Here, we addressed the problem of accurate structural validation with cryo-EM-based methodologies for determining the structures of up to megadalton-scale DNA objects in solution, together with molecular-dynamics-based methods for building pseudoatomic models in a semiautomated fashion. The library of objects includes four brick-like multilayer DNA origami objects with increasing internal floppiness, a barrel-like 126-helix bundle, two variants of a multidomain object called Twisttower, a design variant v2 of a previously reported object called the Pointer, a small 16-helix bundle, four variants of a hinged-beam-like object, two variants of a dumbbell-like object, and five variants of a six-helix tube featuring asymmetric markers at either end as reporters for twist and one ten-helix tube. We constructed pseudoatomic models for six different objects. The fitting was validated using Fourier shell correlation against the cryo-EM half-maps and the models show good cross-correlation with the cryo-EM maps.

The majority of other objects in our library were multilayer DNA origami in honeycomb-lattice packing. Nearly all cryo-EM maps that we determined for objects built using the default seven-base-pair strand crossover spacing prescribed by honeycomb-design rules displayed global right-handed twist deformations (f left, 1 g left, 1 h). The extent of the global twist deformation seen in our panel of honeycomb-lattice structures also decreased with the increasing cross-sectional area, consistent with the behavior we saw for a twist in the domains of the square-lattice Twisttower. The 126-helix bundle, which featured the widest cross section in our panel, did not display any detectable global twist. To show the efficacy of the multibody refinement even when the object does not have clear domains, we applied the multibody approach to three brick-like objects and the 126-helix bundle. Simply dividing the whole object into smaller rigid bodies (right) enabled reconstructing all regions of the objects in greater detail including the peripheries (top vs. bottom).

> TTTTTTTTTGCAATAAAGCCTCAGAGAATTAGCAAAATTAATTTTTTTTT;> TTTTTTTTTAATCATACAGGCAAGGGCATTAACATCCAATATTTTTTTTT;> TTTTTTTTTCAATTCTACTAATAGTGCTGAAAAGGTGGCATTTTTTTTTT;> TTTTTTTTTCAGCTGTGGAGTAGATTAAGATGGCAGGTATGTTTTTTTTT;> TTTTTTTTTTGGGGGCACATGAGTGAGTTTTGGTACCAGGCTTTTTTTTT;> TTTTTTTTTACGAGTAGATTTAGAGTCAACATGTTCTGCGATTTTTTTTT;> TTTTTTTTTTCCCAATTTTAAATATCCATATAACAGTTGATTTTTTTTTT;> TTTTTTTTTCTAATTTTAAGACAAGATGATACAGTGTCTAGTTTTTTTTT;> TTTTTTTTTGCGGGCGCTAGGGCGCGAAGAAAGCGAAAGGATTTTTTTTT;> TTTTTTTTTCACCAGAACCCCAGCTGGCTTGTTGTGGAAGTTTTTTTTTT;> TGTCTAATGTATGGACAGTGGATAAACACGCGCCCTGTAGCGGCGCATTAAGCGCGGCGGGTGTGGTGGTTACGCGCAGCGTGACCGCTACACTTGCCAGCGCCCTAGCGCCCGCTCCTTTCGCTTTCTTCCCTTCCTTTCTCGCCACGTTCGCCGGCTTTCCCCGTCAAGCTCTAAATCGGGGGCTCCCTTTAGGGTTCCGATTTAGTGCTTTACGGCACCTCGACCCCAAAAAACTTGATTTGGGTGATGGTTCACGTAGTGGGCCATCGCCCTGATAGACGGTTTTTCGCCCTTTGACGTTGGAGTCCACGTTCTTTAATAGTGGACTCTTGTTCCAAACTGGAACAACACTCAACCCTATCTCGGGCTATTCTTTTGATTTATAAGGGATTTTGCCGATTTCGGGTAGAATTGGTAAAGAGAGTCGTGTAAAATATCGAGTTCGCACATCTTGTTGTCTGATTATTGATTTTTGGCGAAACCATTTGATCATATGACAAGATGTGTATCTACCTTAACTTAATGATTTTGATAAAAATCATTATAATGCCAGGGTCAGTGAGATGTAACACTACAGACCTCAGCTTCCTCTACTTTGCCTGGCATAGCCTACTGCACCATCCTTTTCAATGGAAGTAATTTGTCCCCCATGGGTTACACCCCCACCTAGACTACTTAAGAAGGTGCTATTGCTCCTGATTTCCAATGTTTGAATCTCCCTCCCACCATACCAGGCATAAAGGCTGTCACTCCCCAATACTAAGTGGCCCCAAGTTCACCACAATACAGCCAAGTGCATTGTTATCACATTCAGTCAAAGAATTTTCATTGGCAACAGTCCTCTCCAATCTGCCTATTCACTGTCCCTACATCAGGTGATAGTCCAGTTGTCAGACATGTGATCCCTGTTTGGGGACCCACAAGGCCTATCCAACCCATTGCTTTTAAAAGAGCTGGGGTTCTGGTGACTTCCACAACAAGCCCATCTGCTCTTAGTACAGCTTGTCTTAAAATTAGCTAGACACTGTATCATACCCCCTCCACTGCCCTATGATAAGGACAGCAGAGGGTTAGATTTACTTATCTGCACTCATGTGCCCCCAGCCTGGTACCAAAACTGATAATCTACTCCACAGCTGCATACCTGCCATCTTAGCCAAACCACACCAATCCAATTGCTGGGTCTCATATCATCTCTGAAGAAGTGATTACCTCATTACATGCTTGCTTGATATACCCACTTTCCTTATGAGGCACACCCATACTGAGGTAGCTATTTTACTATTGACTGGGTAAGCCAGTACAAAATAATCATAGGTGCACAGTCTGGACATGGGAACCCCTCTTCCTACTCACCTCTCTCAGAGGCAATGCCCCTTCATTAACCATGCACCCTAGGCCTTGGTACAAGTTGCCAACCTGCAGAGAACCAGTTAGCTGAAAGGCCAGGTTCTTCTTGATCTTGGTGCTTAGGGCAAACTTTTGGGATAGGCAAAAACAAGTCCTTTACACACCTCCAGTCTACAGTTCCATCAAAGTGGAACTTGGAATGTTATAAACTGCATCTATACTGTACTGCTAGTAGGCTTGTTTAATGCTTTCAACTCCTAGAGAATCACTTCAATCCTACCAACCAATAGTTCCCCATCACACAGATGGCTAAAGACCCTACCTCCCCTAAAGCCCTACTTCACACTGCAGGGACCTCCTAAGGGTCTTGGACCCTCCTCACTTGTTACTAGGCTATCATTCTACTGGTGCAGATACAGATTTTAGGTACCTGTCCTTGATGCACTTAGCTTTAACATGTCACATGCCAATGAAAATAGCAGCCACAGGGGGATATTCTAGGAGCAACATGGAGACTGTCTGCTACAACCACCAAACAGCTCATCCTCTGCATGAATACTTACTCTAGACCCCTGCATTCACCTTCCATGATTAATCACCAACTGAGTCTTGCAAAACCCAATTATGGTTATAGACAGACTGGCCCATGTTACCACTTAAACTCCATCTAGTCTGCAGTGTTCTGACCTATGCCTGAGGGTCCAGATAACCACTCTTCACTAAGCCCCCTGGAAGACAGTTAAGTCTATCTATCAGCCTCACATCCATCCCATTCTCTCTTTGAGATCTTATCAGGACTGATTGTATGTGAACAATATACTCCCAGGCTGGCCATTAGAGATTGGTTAGTGGTTGGCTGGACCAACACCCTTAAGCAACTAATAAGACCATGTGGGGTGTCCAGGCCTCATAAATCCTGAGCCTCTCAATCTTCCAGTGGCTCACCATTCCCATCCACACAACCTATTGGAACCATCAGAGTCATCACCTATATAGGGTGAAGTAGAGCTCCACCACCCCATAACTATACAGTGCACCTGGCCTCTGAGACTTGCTGTGATAACACAAACCCCAGGGCCAAATTGGGAAGATGCAATGACATTCCATTACTTCTCCAGGACAACATTTATTTGTTGCTGACTCCAGACTTAACAAGGAGTATTTGAGGCCACTGTTGGGGCCCTAACCCACCCAGCTCTTGACAGCTAATCTTAACCTCAAGGATTGACCATTGGGGGAGTCAACCAGCTTTGGCCCTGCTCAAGCAAACAATCCCCAGATGACCTGCTGGCAGGCACCCCTAGAAATATTGTGGGTTGCACTATTTCTTGCTCAGATGCTTCCCACTATAGCCCCACTCCAACTAGTACCACATCATTTTATGGATCAATCACAAAGGAGCCCCTATAGGCTGATTCTGTGTTTCAAAAAGTGAAGCCTATGTGCTCCATTGAGTCAGTAAATTAACACCACTAGAAGTTATCCAGCTAGTCAAGGGTTTTCCATATGTCCCAAGGTACTAGCTACAGCACTTGAATATGGTCTACTATGAGTGGGACTATTAATGTCATCTTTCTGTATAGCTGCCCCATTTAAAGCATATATGAAGTGCTAACATTGTGTTGGATCTTTATGCCACCAGATCCCCCTTACAGTATTCTCACCCAAATGGGATGAGAGTTGTATTAAGGCTAGTTAATCCCTAAGTCCATACATAGGACCACAGTAGCTTGGCTATGCTCACAATTTGCCATGTATATCAGTCCCAGAGGTATGCAAGACATTGCCCACATTTCAGAATGGTCCTGTCTTGTGGTTCCTTGCCTTTTGCACATTACCCTTGGCCTTCTACATAATGTGAGTCCTGGCTGCAATCTATGTATTGAAAGTAGGTAACCCTTCTCATTGTCAAGAACATCTGTTCCTAGCCACCCTGACCCTGCCTCCCTGAAGCTGCTCCCATAGGCCCACTGATCTCACTGCTTCTAATTGCATCCCTTGACTCTCTATCCCCTGAGAATTCCTGCTTGTGCAGCCTTGTGAGCCACTACCCAGTCAGGGTGTTAAGCCTTACCATGACCAGGTGCCCTCTATGACTAGCCCAAGACTCACAGACAGGATAGCCAGCTGTACCCCACACTCCTCTTGCCCTGGGCACTCTCATCAGTACCCTCAATAACCTAGCTGTCCACTCACTATCCTCAGACCAATTCTCCTTCTGCCAAAGGTCCAACATAGAGGACTCATCTGGGCTCAGGCAACTCAGGGCATATGGGACCATAGCTCAACTACAATAAAACCAGGGGCCACATAAGCTAGCAATCAGTGGGTGTAAGTGTCTGGGTGCATCAGCTGGTAAGACTGCCAGATTCTATGCAGGCCAATCATGAACCTACTAGTCCCTCATGGTCACTTTGTTCATCTAACAGATAGTTGCTTCAAACTCAAGACCTTACTAACCTTAGTCACTGGTTCTACCAGCCCAGGAATCCTCCTTGGGCTAGCCTCCAAGAAGCTTCAGACTCCTTAATACCAAGCAGCAGGAACAGTTTCAGCACCAAGAGGTGAGAACTGCTGTTAGCATCACTGACTTACAATCTCATGATAGCTAAGCATTCTTAGAACTCTTATATAACTCCCTATTACCAGAGACAGCCCTCAGGATTACTGATGGACCTTCTTCAAGTCTTTTCTAGCACAGGACCTACAGGGAGAGGGAAAGTCAGCTCCTATGGGGAATACAAGAGTTAGTCTTCAGTTTGTGGCTGAGGCTTCTTTGTGCTGGTTGCCTCTAAGACAAATTATTCTGGAATCTAATCAAGTTTACAAGGTCAGCATTATGACCCAGGTCAATAGCTTCTGGGAGGCTCTTCTAGTTTCCACCTTTGTACCAGTATCCTATTTAAGATAGGTCATGCATAGGGCTCTACACAATGAGTTCAGAGCCTTTGCAGCTTAAGGAAATCTCTCCTCCATAAAAGTTCTGCTTTGATGTCAATTCCCCTTGTACTTCCTGTGACTGCAACACAGTTGGACTGGTATTCCTCAACATCAACAATTAGTAAAAGCAATGGTTGTGACCAAGGAATGAGACCAGCAATTAATTGACATAGTTTAACTGTCAAACACTGAGAGATGGAGCCTGCAAGTGGGGCTTATCCCACAGAGTACTGTTTTCTGAGGAGCTGAGTTAACAGGTGGAGAAAATCCCAAAGATACTCTCCCAATGGCCAGTCCAAGCTTGAAGTCAATGCAACCTCTAGTAATAGGTAGAGGCTGCCACAAATGATGCCTACAAAGAGTAAACTTCTATATGTGGTAATGGCATCCAAGTAAAGGGCTAATGCAGAACAGAGCTTTTGTTAATGGGCAAGCTACTACTAAACCCTCTGGAGCATGTGTTAGTAGATACCTTCAACCTTGGAGCTCACTCAGAAAAAGCCTGAACCCAGAATTAAAACATCCTGGTGTACTCTGGCACCAGTGACACCATGGCTTTTTCAGGCCCCTGTGCCTGTTGCATGCAAACCTAAGAGTCTAAAGGTAATCTGTCAGCCAGGAGAGTGGTCTCCATGCCTCAGTGTGTAGGTGGGCAGTCATTCCTATACCATATAAAATGGAGTACATCTACAAGCACTGGACTACCTAGGTTTCCTGGATAGTAACTCTAACCAGACACACATGGCCTGGAGTGGAGTTACCCAACAGAACCCTGTCATATTTCCTAATCCACTAAAGTCTGTTACATACAGGCAGTTTTTGCTCTCTGCTGCCTGCCCAGCAGCTATGGTGATCAACTGGCTAGAATGACTTGTGTACCTACCCTAATTTTAATTTCACTCTGACATGCAGTTCAACAGGCTACCCCTTTTTATTGGTGGCTACATTTGGCTTAATTCTAACTGGTCAGAGATAAAGCTCAGCAGTGATATGAGCCCTTAGGAAAATTCCAGAGCACACACTAGCAGATGTTTTATCATGGAATATTATCAATGTAGCTCTGGGGGTAACTTTGAAAAGCTGTTCACTTACCTTTCCAGGGATAACTTGCATTTAGACATACTAGATTATCTTACATTCTGATATCACTAGTGTCCTGAAACAGGGCTTCATCATAATCCTTGTCACCTGTTAAACCTTTTATATGCCCTTGCTAGGGCCCAACTCTGTCTCCTGTAAAGTTAAAGTGCCTTCAGGAAGTTGGTGAGTAGACCTGAATAATTCATACTTTATCTCCTACACCAGGATGACTCAGTAGGACATCTCAGTCTCTAATACTCATACAAATACACTCTATTAGGGGCTGGGACACCTGATCCAGAAACAAAGTTTCTTAAGTACCTCTGTACAATTGAAGATAATGGTACTCAATGATATTTTGTGATTCAAATTTACAGAGAGCAGTAATGTTCCCAGTTTATCCTTAGATAGAGCAAAAGATTAAAGAACCTGGTTAATATTTAGGATCTGATGATCCTGCACACTTCTGAATGCCTTGAAATTCTTGTCCATTCAATACCCTGGTCTTAGGCCATATCCTGTTCTAGAACACTTATGCACAATCAATATGCATGGGCTGTGTGAGGGCTGCTATCTGTAGGCACTAATGGATTTGTAAGCTGGCTCTGTTTCTCTTACTTTCAGTATACCTATCAAGGTTTTGGTGTTGAAACCTGACTGACCACTGGCAAAGGGTGGGAAACTTAGGTTCCCTAGTATGCTAGCTTAGCAACCATAAGGTCTATTGTCTCAAATCAAAATCTAGGGGAACATGATCTGGATGCCCATATTCAAGCCAACAAATCTTGAACTGGGATTCCAAGGGCCTAACAACTATTCCACTTGGCACTTTAGCAGGCTCATTCATGCTCTGATCAGTTGCAATTTATGAAACTGTAGTCTCAGGTCCTAGGAATTATAGGTTGTACACTGGGCCTCCTGGGAATTGTTTGCTACTTGACCTCTTTCATGTACATGTTGATGGGGTAGTACTAATTAAGAGCCATAGTCATAAGTAGTTGGGCATGCTGAATCATCCAGTAGAAGGCTCCAGCATGAGGTGGCATTGATGAACAGCCTAAGCTTATTGCAAGCATGGCACATAGCACCTAACTTCATGACTGTTATTCATTTACCTGAGTATAGGATTTCATATAGATCCAAATAGGAACTAAGGTTCATAGTAGCCATCATGTTCAAAGCTATAACAAACATTAAATATATCCATGTCCTAAATGCATTAGGTGAACCAAGTCACAGGTACAGAAAGGGGATGCAGCACAAAAATTGATACTTGTAGAAAGAGGATTCAGATATATTGAGCTGTGCTACCATTAATAAAGATGGGTCCCATGAAGAGCATCTTCTGTTGTTAGGTCTGACTATGGCAGCAAATCCAGGTAAGGCAAGGACTAGTTCTCAAGTGACCTTTAAGTTGACTTTTAGCCTGTATTTCAAGGCTTAGAGGGCACAACTGTGTCTATAAATTGCCTAATGAATCCATAGACTTTACCAATGCTGTCTAGATATGCTTAAAGGAAGAGTGTTGTAGTGTATGAACTTTCTATTTGCTGCTGAGATATTAGTTGTGGATCCTAGTTGAATTTCTAAGTTAGGCAGGTATCTGGCTTGCAGGATCCATTTCTGCAAAGTAAGAGGGGGTCATTGCAGACCCATGCTATGTCTGTGAAAGATCTGTGCATATCTAGAGGTTAGGACTTCAGCTACCTGGGTTTGCATAAGAATAAGCAGACTAAAAGGCATGACAGAAGACTTCTTATGGGTAGCAGTCTTATTTTTAGAGTTCTTGGGAGATCAGATCTAAGGAGATTCACAAGAAACTAGAGTAGCATTGGAGATGAGTAACATATACACATATTACTACATGGTTTACTGCCTTAAATGTGGCCTAGGGTATTATGCTGGAGAGCTAGGTGTCAGTTCTAAAAAGGATAAGTCATGGGGGCCTTTCACAGCAAGTTACAAACTATGTTTAGTATCAGAACTTATTAAACATAACAGTAACCAAAGCCATGGTATGATGTACTATCTTTTTGTAGCACTAGGATACTATATTAACTACTCTTTAGTTTTGTCATGAGAAGTACACCTTATAGCATAGATTGAATGGGTGGATGTCTCTGTGGAGGTGTGTGCTTGGATTAGATGGTGTGAATAGAAAACTAAATACTGGATTGGACAAGTGTT;> TTAAGCTCTAAGCCATCCGCAAAAATGACCTCTTATCAAAAGGAGCAATTAAAGGTACTCTCTAATCCTGACCTGTTGGAGTTTGCTTCCGGTCTGGTTCGCTTTGAAGCTCGAATTAAAACGCGATATTTGAAGTCTTTCGGGCTTCCTCTTAATCTTTTTGATGCAATCCGCTTTGCTTCTGACTATAATAGTCAGGGTAAAGACCTGATTTTTGATTTATGGTCATTCTCGTTTTCTGAACTGTTTAAAGCATTTGAGGGGGATTCAATGAATATTTATGACGATTCCGCAGTATTGGACGCTATCCAGTCTAAACATTTTACTATTACCCCCTCTGGCAAAACTTCTTTTGCAAAAGCCTCTCGCTATTTTGGTTTTTATCGTCGTCTGGTAAACGAGGGTTATGATAGTGTTGCTCTTACTATGCCTCGTAATTCCTTTTGGCGTTATGTATCTGCATTAGTTGAATGTGGTATTCCTAAATCTCAACTGATGAATCTTTCTACCTGTAATAATGTTGTTCCGTTAGTTCGTTTTATTAACGTAGATTTTTCTTCCCAACGTCCTGACTGGTATAATGAGCCAGTTCTTAAAATCGCATAAGGTAATTCACAATGATTAAAGTTGAAATTAAACCATCTCAAGCCCAATTTACTACTCGTTCTGGTGTTTCTCGTCAGGGCAAGCCTTATTCACTGAATGAGCAGCTTTGTTACGTTGATTTGGGTAATGAATATCCGGTTCTTGTCAAGATTACTCTTGATGAAGGTCAGCCAGCCTATGCGCCTGGTCTGTACACCGTTCATCTGTCCTCTTTCAAAGTTGGTCAGTTCGGTTCCCTTATGATTGACCGTCTGCGCCTCGTTCCGGCTAAGTAACATGGAGCAGGTCGCGGATTTCGACACAATTTATCAGGCGATGATACAAATCTCCGTTGTACTTTGTTTCGCGCTTGGTATAATCGCTGGGGGTCAAAGATGAGTGTTTTAGTGTATTCTTTTGCCTCTTTCGTTTTAGGTTGGTGCCTTCGTAGTGGCATTACGTATTTTACCCGTTTAATGGAAACTTCCTCATGAAAAAGTCTTTAGTCCTCAAAGCCTCTGTAGCCGTTGCTACCCTCGTTCCGATGCTGTCTTTCGCTGCTGAGGGTGACGATCCCGCAAAAGCGGCCTTTAACTCCCTGCAAGCCTCAGCGACCGAATATATCGGTTATGCGTGGGCGATGGTTGTTGTCATTGTCGGCGCAACTATCGGTATCAAGCTGTTTAAGAAATTCACCTCGAAAGCAAGCTGATAAACCGATACAATTAAAGGCTCCTTTTGGAGCCTTTTTTTTGGAGATTTTCAACGTGAAAAAATTATTATTCGCAATTCCTTTAGTTGTTCCTTTCTATTCTCACTCCGCTGAAACTGTTGAAAGTTGTTTAGCAAAATCCCATACAGAAAATTCATTTACTAACGTCTGGAAAGACGACAAAACTTTAGATCGTTACGCTAACTATGAGGGCTGTCTGTGGAATGCTACAGGCGTTGTAGTTTGTACTGGTGACGAAACTCAGTGTTACGGTACATGGGTTCCTATTGGGCTTGCTATCCCTGAAAATGAGGGTGGTGGCTCTGAGGGTGGCGGTTCTGAGGGTGGCGGTTCTGAGGGTGGCGGTACTAAACCTCCTGAGTACGGTGATACACCTATTCCGGGCTATACTTATATCAACCCTCTCGACGGCACTTATCCGCCTGGTACTGAGCAAAACCCCGCTAATCCTAATCCTTCTCTTGAGGAGTCTCAGCCTCTTAATACTTTCATGTTTCAGAATAATAGGTTCCGAAATAGGCAGGGGGCATTAACTGTTTATACGGGCACTGTTACTCAAGGCACTGACCCCGTTAAAACTTATTACCAGTACACTCCTGTATCATCAAAAGCCATGTATGACGCTTACTGGAACGGTAAATTCAGAGACTGCGCTTTCCATTCTGGCTTTAATGAGGATTTATTTGTTTGTGAATATCAAGGCCAATCGTCTGACCTGCCTCAACCTCCTGTCAATGCTGGCGGCGGCTCTGGTGGTGGTTCTGGTGGCGGCTCTGAGGGTGGTGGCTCTGAGGGTGGCGGTTCTGAGGGTGGCGGCTCTGAGGGAGGCGGTTCCGGTGGTGGCTCTGGTTCCGGTGATTTTGATTATGAAAAGATGGCAAACGCTAATAAGGGGGCTATGACCGAAAATGCCGATGAAAACGCGCTACAGTCTGACGCTAAAGGCAAACTTGATTCTGTCGCTACTGATTACGGTGCTGCTATCGATGGTTTCATTGGTGACGTTTCCGGCCTTGCTAATGGTAATGGTGCTACTGGTGATTTTGCTGGCTCTAATTCCCAAATGGCTCAAGTCGGTGACGGTGATAATTCACCTTTAATGAATAATTTCCGTCAATATTTACCTTCCCTCCCTCAATCGGTTGAATGTCGCCCTTTTGTCTTTGGCGCTGGTAAACCATATGAATTTTCTATTGATTGTGACAAAATAAACTTATTCCGTGGTGTCTTTGCGTTTCTTTTATATGTTGCCACCTTTATGTATGTATTTTCTACGTTTGCTAACATACTGCGTAATAAGGAGTCTTAATCATGCCAGTTCTTTTGGGTATTCCGTTATTATTGCGTTTCCTCGGTTTCCTTCTGGTAACTTTGTTCGGCTATCTGCTTACTTTTCTTAAAAAGGGCTTCGGTAAGATAGCTATTGCTATTTCATTGTTTCTTGCTCTTATTATTGGGCTTAACTCAATTCTTGTGGGTTATCTCTCTGATATTAGCGCTCAATTACCCTCTGACTTTGTTCAGGGTGTTCAGTTAATTCTCCCGTCTAATGCGCTTCCCTGTTTTTATGTTATTCTCTCTGTAAAGGCTGCTATTTTCATTTTTGACGTTAAACAAAAAATCGTTTCTTATTTGGATTGGGATAAATAATATGGCTGTTTATTTTGTAACTGGCAAATTAGGCTCTGGAAAGACGCTCGTTAGCGTTGGTAAGATTCAGGATAAAATTGTAGCTGGGTGCAAAATAGCAACTAATCTTGATTTAAGGCTTCAAAACCTCCCGCAAGTCGGGAGGTTCGCTAAAACGCCTCGCGTTCTTAGAATACCGGATAAGCCTTCTATATCTGATTTGCTTGCTATTGGGCGCGGTAATGATTCCTACGATGAAAATAAAAACGGCTTGCTTGTTCTCGATGAGTGCGGTACTTGGTTTAATACCCGTTCTTGGAATGATAAGGAAAGACAGCCGATTATTGATTGGTTTCTACATGCTCGTAAATTAGGATGGGATATTATTTTTCTTGTTCAGGACTTATCTATTGTTGATAAACAGGCGCGTTCTGCATTAGCTGAACATGTTGTTTATTGTCGTCGTCTGGACAGAATTACTTTACCTTTTGTCGGTACTTTATATTCTCTTATTACTGGCTCGAAAATGCCTCTGCCTAAATTACATGTTGGCGTTGTTAAATATGGCGATTCTCAATTAAGCCCTACTGTTGAGCGTTGGCTTTATACTGGTAAGAATTTGTATAACGCATATGATACTAAACAGGCTTTTTCTAGTAATTATGATTCCGGTGTTTATTCTTATTTAACGCCTTATTTATCACACGGTCGGTATTTCAAACCATTAAATTTAGGTCAGAAGATGAAATTAACTAAAATATATTTGAAAAAGTTTTCTCGCGTTCTTTGTCTTGCGATTGGATTTGCATCAGCATTTACATATAGTTATATAACCCAACCTAAGCCGGAGGTTAAAAAGGTAGTCTCTCAGACCTATGATTTTGATAAATTCACTATTGACTCTTCTCAGCGTCTTAATCTAAGCTATCGCTATGTTTTCAAGGATTCTAAGGGAAAATTAATTAATAGCGACGATTTACAGAAGCAAGGTTATTCACTCACATATATTGATTTATGTACTGTTTCCATTAAAAAAGGTAATTCAAATGAAATTGTTAAATGTAATTAATTTTGTTTTCTTGATGTTTGTTTCATCATCTTCTTTTGCTCAGGTAATTGAAATGAATAATTCGCCTCTGCGCGATTTTGTAACTTGGTATTCAAAGCAATCAGGCGAATCCGTTATTGTTTCTCCCGATGTAAAAGGTACTGTTACTGTATATTCATCTGACGTTAAACCTGAAAATCTACGCAATTTCTTTATTTCTGTTTTACGTGCAAATAATTTTGATATGGTAGGTTCTAACCCTTCCATTATTCAGAAGTATAATCCAAACAATCAGGATTATATTGATGAATTGCCATCATCTGATAATCAGGAATATGATGATAATTCCGCTCCTTCTGGTGGTTTCTTTGTTCCGCAAAATGATAATGTTACTCAAACTTTTAAAATTAATAACGTTCGGGCAAAGGATTTAATACGAGTTGTCGAATTGTTTGTAAAGTCTAATACTTCTAAATCCTCAAATGTATTATCTATTGACGGCTCTAATCTATTAGTTGTTAGTGCTCCTAAAGATATTTTAGATAACCTTCCTCAATTCCTTTCAACTGTTGATTTGCCAACTGACCAGATATTGATTGAGGGTTTGATATTTGAGGTTCAGCAAGGTGATGCTTTAGATTTTTCATTTGCTGCTGGCTCTCAGCGTGGCACTGTTGCAGGCGGTGTTAATACTGACCGCCTCACCTCTGTTTTATCTTCTGCTGGTGGTTCGTTCGGTATTTTTAATGGCGATGTTTTAGGGCTATCAGTTCGCGCATTAAAGACTAATAGCCATTCAAAAATATTGTCTGTGCCACGTATTCTTACGCTTTCAGGTCAGAAGGGTTCTATCTCTGTTGGCCAGAATGTCCCTTTTATTACTGGTCGTGTGACTGGTGAATCTGCCAATGTAAATAATCCATTTCAGACGATTGAGCGTCAAAATGTAGGTATTTCCATGAGCGTTTTTCCTGTTGCAATGGCTGGCGGTAATATTGTTCTGGATATTACCAGCAAGGCCGATAGTTTGAGTTCTTCTACTCAGGCAAGTGATGTTATTACTAATCAAAGAAGTATTGCTACAACGGTTAATTTGCGTGATGGACAGACTCTTTTACTCGGTGGCCTCACTGATTATAAAAACACTTCTCAGGATTCTGGCGTACCGTTCCTGTCTAAAATCCCTTTAATCGGCCTCCTGTTTAGCTCCCGCTCTGATTCTAACGAGGAAAGCACGTTATACGTGCTCGTCAAAGCAACCATAGTACGCGCCCTGTAGCGGCGCATTAAGCGCGGCGGGTGTGGTGGTTACGCGCAGCGTGACCGCTACACTTGCCAGCGCCCTAGCGCCCGCTCCTTTCGCTTTCTTCCCTTCCTTTCTCGCCACGTTCGCCGGCTTTCCCCGTCAAGCTCTAAATCGGGGGCTCCCTTTAGGGTTCCGATTTAGTGCTTTACGGCACCTCGACCCCAAAAAACTTGATTTGGGTGATGGTTCACGTAGTGGGCCATCGCCCTGATAGACGGTTTTTCGCCCTTTGACGTTGGAGTCCACGTTCTTTAATAGTGGACTCTTGTTCCAAACTGGAACAACACTCAACCCTATCTCGGGCTATTCTTTTGATTTATAAGGGATTTTGCCGATTTCGGAACCACCATCAAACAGGATTTTCGCCTGCTGGGGCAAACCAGCGTGGACCGCTTGCTGCAACTCTCTCAGGGCCAGGCGGTGAAGGGCAATCAGCTGTTGCCCGTCTCACTGGTGAAAAGAAAAACCACCCTGGCGCCCAATACGCAAACCGCCTCTCCCCGCGCGTTGGCCGATTCATTAATGCAGCTGGCACGACAGGTTTCCCGACTGGAAAGCGGGCAGTGAGCGCAACGCAATTAATGTGAGTTAGCTCACTCATTAGGCACCCCAGGCTTTACACTTTATGCTTCCGGCTCGTATGTTGTGTGGAATTGTGAGCGGATAACAATTTCACACAGGAAACAGCTATGACCATGATTACGAATTCGAGCTCGGTACCCGGGGATCCTCCGTCTTTATCGAGGTAACAAGCACCACGTAGCTTAAGCCCTGTTTACTCATTACACCAACCAGGAGGTCAGAGTTCGGAGAAATGATTTATGTGAAATGCGTCAGCCGATTCAAGGCCCCTATATTCGTGCCCACCGACGAGTTGCTTACAGATGGCAGGGCCGCACTGTCGGTATCATAGAGTCACTCCAGGGCGAGCGTAAATAGATTAGAAGCGGGGTTATTTTGGCGGGACATTGTCATAAGGTTGACAATTCAGCACTAAGGACACTTAAGTCGTGCGCATGAATTCACAACCACTTAGAAGAACATCCACCCTGGCTTCTCCTGAGAAAGCTTGGCACTGGCCGTCGTTTTACAACGTCGTGACTGGGAAAACCCTGGCGTTACCCAACTTAATCGCCTTGCAGCACATCCCCCTTTCGCCAGCTGGCGTAATAGCGAAGAGGCCCGCACCGATCGCCCTTCCCAACAGTTGCGCAGCCTGAATGGCGAATGGCGCTTTGCCTGGTTTCCGGCACCAGAAGCGGTGCCGGAAAGCTGGCTGGAGTGCGATCTTCCTGAGGCCGATACTGTCGTCGTCCCCTCAAACTGGCAGATGCACGGTTACGATGCGCCCATCTACACCAACGTGACCTATCCCATTACGGTCAATCCGCCGTTTGTTCCCACGGAGAATCCGACGGGTTGTTACTCGCTCACATTTAATGTTGATGAAAGCTGGCTACAGGAAGGCCAGACGCGAATTATTTTTGATGGCGTTCCTATTGGTTAAAAAATGAGCTGATTTAACAAAAATTTAATGCGAATTTTAACAAAATATTAACGTTTACAATTTAAATATTTGCTTATACAATCTTCCTGTTTTTGGGGCTTTTCTGATTATCAACCGGGGTACATATGATTGACATGCTAGTTTTACGATTACCGTTCATCGATTCTCTTGTTTGCTCCAGACTCTCAGGCAATGACCTGATAGCCTTTGTAGATCTCTCAAAAATAGCTACCCTCTCCGGCATTAATTTATCAGCTAGAACGGTTGAATATCATATTGATGGTGATTTGACTGTCTCCGGCCTTTCTCACCCTTTTGAATCTTTACCTACACATTACTCAGGCATTGCATTTAAAATATATGAGGGTTCTAAAAATTTTTATCCTTGCGTTGAAATAAAGGCTTCTCCCGCAAAAGTATTACAGGGTCATAATGTTTTTGGTACAACCGATTTAGCTTTATGCTCTGAGGCTTTATTGCTTAATTTTGCTAATTCTTTGCCTTGCCTGTATGATTTATTGGATGTTAATGCTACTACTATTAGTAGAATTGATGCCACCTTTTCAGCTCGCGCCCCAAATGAAAATATAGCTAAACAGGTTATTGACCATTTGCGAAATGTATCTAATGGTCAAACTAAATCTACTCGTTCGCAGAATTGGGAATCAACTGTTATATGGAATGAAACTTCCAGACACCGTACTTTAGTTGCATATTTAAAACATGTTGAGCTACAGCATTATATTCAGCAAT;> TTTTTTTTTTGAGTGTTGTTCCAGTTAGCCCGAGATAGGGTTTTTTTTTT;> TTTTTTTTTGGGAAGAAAGCGAAAGCGTGGCGAGAAAGGAATTTTTTTTT;> TTTTTTTTTAAGTGTTTTTATAATCACGCCAGAATCCTGAGTTTTTTTTT;> TTTTTTTTTAATGGATTATTTACATACGCTCAATCGTCTGATTTTTTTTT;> TTTTTTTTTAATTTACTGACTCAATAACTTCTAGTGGTGTTTTTTTTTTT;> TTTTTTTTTCACAGAATCAGCCTGAGCTTCACTTTTTGAAATTTTTTTTT;> TTTTTTTTTGTGATTGATCCATATAGTATAGGGGCTCCTTTTTTTTTTTT;> TTTTTTTTTTAGTTGGAGTGGGGCAATAAATGATGTGGTACTTTTTTTTT;> TTTTTTTTTATCTGAGCAAGAAATTCTCTATAGTGGGAAGCTTTTTTTTT;> TTTTTTTTTATATTTCTAGGGGTGCGGTAGTGCAACCCACATTTTTTTTT;> TTTTTTTTTGATTGTTTGCTTGAGCCAGCAGGTCATCTGGGTTTTTTTTT;> TTTTTTTTTCCCCCAATGGTCAATCCCAAAGCTGGTTGACTTTTTTTTTT;> TTTTTTTTTTCAAGAGCTGGGTGGGAGGTTAAGATTAGCTGTTTTTTTTT;> TTTTTTTTTTCAAATACTCCTTGTTGGCCCCAACAGTGGCCTTTTTTTTT;> TTTTTTTTTGCCTTGAATCGGCTGAGGGCACGAATATAGGGTTTTTTTTT;> TTTTTTTTTTCTGTAAGCAACTCGTCAGTGCGGCCCTGCCATTTTTTTTT;> TTTTTTTTTGAGTGACTCTATGATAATTTACGCTCGCCCTGTTTTTTTTT;> TTTTTTTTTAATAACCCCGCTTCTAGACAATGTCCCGCCAATTTTTTTTT;> TTTTTTTTTTGCTGAATTGTCAACCATTTAAGTGTCCTTAGTTTTTTTTT;> TTTTTTTTTTTCATGCGCACGACAAATTAAGTGGTTGTGAATTTTTTTTT;> TTTTTTTTTGGTGGATGTTCTTCTTAATCAGGAGAAGCCAGTTTTTTTTT;> TTTTTTTTTAGTGCCAAGCTTTCGGTAGTAAAACGACGGCCTTTTTTTTT;> TTTTTTTTTCCAGTCACGACGTTGCCAACGCCAGGGTTTTCTTTTTTTTT;> TTTTTTTTTCAACCACTAACCAAACCTGGTGTTGGTCCAGCTTTTTTTTT;> TTTTTTTTTCCTGGGAGTATATTCATATCTCTAATGGCCAGTTTTTTTTT;> TTTTTTTTTAGTCCTGATAAGATTCCAGTTCACATACAATCTTTTTTTTT;> TTTTTTTTTGGGATGGATGTGAGGCTCCTCAAAGAGAGAATTTTTTTTTT;> TTTTTTTTTCTTCCAGGGGGCTTAGAGATAGACTTAACTGTTTTTTTTTT;> TTTTTTTTTCCTCAGGCATAGGTCAGAGTGGTTATCTGGACTTTTTTTTT;> TTTTTTTTTAGTTTAAGTGGTAACAACTGCAGACTAGATGGTTTTTTTTT;> TTTTTTTTTCATAATTGGGTTTTGCCCAGTCTGTCTATAACTTTTTTTTT;> TTTTTTTTTAGGTGAATGCAGGGGCGGTGATTAATCATGGATTTTTTTTT;> TTTTTTTTTTTCATGCAGAGGATATAAGTCTAGAGTAAGTATTTTTTTTT;> TTTTTTTTTTTGTAGCAGACAGTCAATGAGCTGTTTGGTGGTTTTTTTTT;> TTTTTTTTTTAGAATATCCCCCTGTCCCTCCATGTTGCTCCTTTTTTTTT;> TTTTTTTTTTGTGACATGTTAAAGCGCTATTTTCATTGGCATTTTTTTTT;> TTTTTTTTTACCTAAAATCTGTATCTGCATCAAGGACAGGTTTTTTTTTT;> TTTTTTTTTCTAGTAACAAGTGAGGCCAGTAGAATGATAGCTTTTTTTTT;> TTTTTTTTTAAAGCCCCAAAAACAGCCGGTTGATAATCAGATTTTTTTTT;> TTTTTTTTTGCATGTCAATCATATGGGTAATCGTAAAACTATTTTTTTTT;> TTTTTTTTTAAACAAGAGAATCGATCCTGAGAGTCTGGAGCTTTTTTTTT;> TTTTTTTTTCAAAGGCTATCAGGTCTTTTTTGAGAGATCTATTTTTTTTT;> TTTTTTTTTGAGAGGGTAGCTATGCAAATAAATTAATGCCGTTTTTTTTT;> TTTTTTTTTAACCGTTCTAGCTGGAAATCAATATGATATTCTTTTTTTTT;> TTTTTTTTTCAGTCAAATCACCAAATGAGAAAGGCCGGAGATTTTTTTTT;> TTTTTTTTTGCCTATCCCAAAAGAACCAAGGACTTGTTTTTTTTTTTTTT;> TTTTTTTTTCAAGATCAAGAAGACCTTTTTGCCCTAAGCACTTTTTTTTT;> TTTTTTTTTCTAACTGGTTCTCTGCGCACCTGGCCTTTCAGTTTTTTTTT;> TTTTTTTTTTGTAATACCCTGACTAGGAAACATTATGACCCTTTTTTTTT;> TTTTTTTTTATCGGTTGTACCAATAACGAGCATAAAGCTAATTTTTTTTT;> TTTTTTTTTATTGTTATCCGCTCACAACAATTCGAATCAATA;> AAAGAAATACATGGCTTTTTTGTATTTGGAGTTGGGTAGCCA;> GGGTCAGAAGGAGCAAGTTTGCAAGGAAGAGCATAAATATCT;> GTTTGAGGCAATTCCAACTCGTCATTAGACTTTACCGATTGG;> GAGAGTCAAGGGATGGGAGCAATTCCTGCCCGAACCATTCTG;> AAGAAATGGTAATATCCAGTAACTGAGAACTTTAAGCCACCA;> TTTTTTTTTGGAGGATCCCCGAACCAATAGGAATTTTTTTTT;> CGCGCAGACACCTATTATTCTGAAACTTTTAAGTTACAAAAT;> TTTTTTTTTACGTGGTGCTTGAAATTTTTGTTATTTTTTTTT;> GAGGATATATCCTGTATTAACAATATCACGGGGAAGCACTAA;> TTTTTTTTTCTTGTGGGTCCCCAAAAATGGGTTGGATAGGCTTTTTTTTT;> TTTTTTTTTACTGGACTATCACCTGGATCACATGTCTGACATTTTTTTTT;> TTTTTTTTTCAGATTGGAGAGGAGGAGGGACAGTGAATAGGTTTTTTTTT;> TTTTTTTTTATGGTGGGAGGGAGATAGCCTTTATGCCTGGTTTTTTTTTT;> TTTTTTTTTAATTCTTTGACTGAATTGCTGTTGCCAATGAATTTTTTTTT;> CACCACACCCGCCGAGCACTAACTCCAGGAAACCTGCAAATAAGCATAT;> CGCCAGCTCTGGCCAGCCCTAGGTGAGGTCCCACTCATAGTAATGTTAG;> CTGATATAACTAATACCCTCATATATGCTTAATAGCGGTCAGTATTAAC;> TACATCGGGAGAAATTTGCACCAGTGCCCGCAGTCATCCTGGACTCACC;> AATTCAATTACCTGGTCGCTATTAATCTGACCTCCTGGTTTTTTTTTTT;> AAACACCGGAAGAGTTCTAAGAATGCATCTTCCCAATTTGTTTTTTTTT;> TGTAAGGTTGACCTACTTTTAACAGGGGAATTGACAAGCTTAGGCTGTT;> GGGTCATCATGCTGTCCTAGGACCTGCTGGAATAATTTGTCTGGGCTGT;> CTGCAAAGGCTCTGCAAAGGTCTTATGAGTAGCAACCAAAAGGAAAGGA;> GCCAGTTACAAAATGTTTTGACTGATAACACCAACCGAGAGGCTTTTAA;> TAACATAAAAACAGGTAATTGAGGACAGATCTTGATACCACAACATAGC;> TTTTTTTTTCAAAGCGCCATTCGCCAAGCAATAGCTAGCAAACGTAGTG;> TTATTTTAAATTATAGAGTGAGGGGTAGGCAAGGCATCGGCAAACAGCT;> TTTTTTTTTGGCGCATCGTAACCAATCACCAGTAGCCGGATAGGTCACG;> TTTTTTTTTTGTTAAAATTCGCAATGAAAGTATTACGCCACCCTCAGAA;> CGTAACAAACTATACCAAGGAGGATTCCAACAGCAACAATAGAGTTGTT;> TCTTTCCAGACGCCGAACCACCCTCATTGAACGCGAGAAAGTCGTAGCT;> AGCATGAATGAGCCCATACTAGGGAAGTGCTTAGCTATCATGTAAGGTT;> CAACCATCTACAGAAGTTTGGATCTATAATGCTTTAAACATACAGCAAA;> TTTGTTATAAAACAGCGAAACCCTCTTTCTTGGATCATTAGACGGGAGA;> ATTTCAAAATCTACAATAAGTGTGTCTGTCGAGGTGATGGCCCACTACG;> AGACTGCGTAAGAGCAACACTTTAGGAACAAGAACCTAGACAAGGGGCC;> TTTTTTTTTCAAGCATGTAATCTCCACTTTGATGGAACTGTTTTTTTTT;> AGAAGTTTTGCCAGCCCTCAATGAAATCGAGGGTAGGCTGTCTGTGTAG;> TTTTTTTTTCAGAGATGATATCATACAGTATAGATGCAGTTTTTTTTTT;> AAGAGTCCACTATTATCGGAAATTAGAGAGCGTCACCACCAGGGTGGCT;> TATTGGGCATTGTGAATTACCAGTCAGGTCAATAGTAACTCCAATCGGA;> GTTTGATCAAAGGGACCCTAAGCGTAACGCGGGAGAACCGTT;> GTCCACGAGTATGTTATCTTAGGAGAAACAATGAAATTCAGT;> TTTTTTTTTTGGCCCTGAGAGAGTTGCAGCAAGCGTGAACCA;> CGAAAAACCGTCTACAGGCGAGATTAAGAAGAAAATGAAAAA;> CGGCGAAGAGCGGGGAACGGTAGTGAGGCATTTTGTGGCAGA;> TTTTTTTTTGGGCAACAGCTGATCAAATCAAGTTTGCGCGTA;> GATTAAAAGTCTGTAAACGCTGACCAGTAAAATACCGAACCC;> GGAGGCCAGCGGTCACGCTGCAGGGAGCAGGGTTCTTGTAGA;> GCTTTCCTTGATTATAATATCCCTTCTGGTCTTTAACCGCCT;> TTTGACGTGCCTGAGTAGACGTATTGGGCGCCATTTTTTTTT;> GTAGCAATACTTCTTCGTTAGTTGACGGGTCACAAACGTTGG;> TTTTTTTTTGGAGAGGCGGTTTGAGAACTCAAACTGAATACG;> TTTTTTTTTCTGCATTAATGAATCAGACAATATTTCTCAGTC;> CAGCAATGCAACAGTGCCACGTTGAATGTCATAGCCACCATT;> GGGGCAGACCTCAAATATCAAAGATTAGCACCACCCCAGCAT;> AGTTGGCCAACACAGACCATAGAAGATAAAACAGAAAACATC;> TTTTTTTTTTAATGAGTGAGCTAACTAGCATCACCAATACAT;> AGCCGTCGCATACCTCTGGGAAAATGTGCAGGTCTTGTAGGA;> GAAGTTTAATAGATTTGCTGACTAATGAAAAATCTTTATTAG;> TTTGCTACCAAGGGGTCCTATAAATTGAGGAAGGTCGCCACC;> GTCAGACCCAGAGCCACTTCAATCAATATCTGGTCTTAGGAG;> TACATTGAGTATGTTTAAGTTAATCAGACAACAAGAAAGAAT;> CGTTTTGTTTTCGGGCTATTAACCTGAAAGCGTAAATCGGCC;> CTCAGGACTAGTGATCTGCTAGTGTGGAGTAAGGGCTCATCC;> GCCACCCATAATCTATAATATAGTTTGCGCCATTAAATAAAA;> CAGAGCCGAACCACAGCCCGAGTGGACTCCAACGTCGAGGTG;> CAAAATCGGCAGGTCACATTAAATGTGAGCGAGTTTTTTTTT;> CCACCCTTTGTTCCAGTTTGGATATCAAATATGGTGGACAAA;> GCCGCCGGGAACCGCAAGTTAGTTACCCTGTAGCGAACTGAT;> AAATCCTAACAGTTAATGCTTGGATGGAAGGGTTAGCTTTGA;> TTTTTTTTTGGTGTAATGAGTACGTTAATATTTTTTTTTTTT;> TTTTTTAAGTTGAGCTAGTAGCTTTTTAACAACTATCTGTTA;> ATATATGTGAGTGAAAACATCGTATCACGAAGGATCTGGAAG;> ATAACCTCACCCACACCAGCTGTCAATAGTGAATTGCTGATG;> CTATGGTAAAACCTGGATATGGTATTCACATTTTTGCGGATG;> TTTTTTTTTACAAATAAATGTTCCAAGACCCTTTTTTTTTTT;> CAAATCCTGAAGCTTCTTGGAGTGCTGATCCCCTACCAGTTC;> TGGGCTGAGGTTGGAGACTACGTTCATGATTGGCCCCTGGTT;> GGCTAGCTGTAAATTATCAAAAATCTGGCAGTCTTTGATTGC;> TTTTTTTTTTGGAATGTCATTGTGAAGTAGGGCTTTTTTTTT;> TTTTTTTTTGCCCTGGGGTTTTCTTTAGCCATCTTTTTTTTT;> ATCCTGATAGAGGCCTATAATGAGCCTTCTTTCATCAATGCC;> TAGGTCCACTAACTAGGTCAACTATGGCCGATATATCGGAAC;> TTTTTTTTTTCTCAGAGGCCAATTGGTTGGTAGTTTTTTTTT;> AGCCTCACCAGGAGAGCATGCCTTGCAGCCTCAGCACAGTCA;> CTTGTATGGCAGAGGCATTTTCATGTTCACTGGTAAACTCAT;> GAGAATCGCCATATATACAGTAGGGCTTAACTGACTTTCCCT;> AAACTTGATTAGATTCCAGTGCACTGTATAGTTTTTTTTTTT;> TAAAGTAACAAAGAAAGGTCCTACTAGATAAGAATTGATGCT;> CGAGCCAACTGAAGTGTGCTATATCATATGTGATACCTCTTG;> CCTTAAGGGGTATTAGCCGTTGTTGATGGGCTCCATGCACCC;> TTTCCTTAGGAATCCAACCATACAGTTAAATCAAGCTAATTT;> TTTTTTTTTATGGGAATGGTGAGCCATCACAGGAAGTACATC;> ATCGAGAACAAGCAAAACCAATCGTCACGGAGTTACTAAACA;> TTTATTTTCATCGTATCATTCGACAGCATTCGGTCCTGTGAA;> TCCAACTGTGGGATCCAGCTCCTCAGAATTCTGTACCTGTAG;> TGCTTTTGAACATGCAGGTAATATTCATAGAACTGACACCTA;> TTGGTCAATTACCGCGCCCAAAATAATCGCAACGGCGCCCAC;> TCATTCCCCTTAGTTCCTATTACGAAGGATTGTGTACCCATC;> AGGCCCAGTACTCTGTGTTGCTGCATTTATGCTTGGAGGCAG;> AGCTACAACCAAGCCTCATCTCTAGTTTGATAGCGTCTAATA;> AACTCTGATCTTTGGGATTTTAAAAGCTCTGCATCAGGTCAC;> TAACGAGTGGACTGGCCATTGCCCTTTACTACAAGTTGCCTT;> CGTCTTTCCAGAGCATTAGTTAACGGAGGCAAAAGTAGATCT;> AGAAATGCATATTATTTATCCGAACCTCCGCGACCTACGTAA;> CATCATTTAGCAGCCTTTACAAGAGATACGAACTGTCATTAC;> TAATTCTGGGTTCACAGGCACGCATTGGCTAATATACTTTGC;> CATGCAAGGCTTTTTCAGAGGGGAAGCGGCCATTATCAAGCT;> GCCATGGTCCTTTAGAAAGTTGAACTAAGAAGAAACTTTAAT;> TGTCACTCCGAAGCCCTTTTTACTCCTTTATCCAGGCCATGT;> ATAACGGCCGAAATCGGCAAAAAAGAACTTAGAGCCAAGTGT;> ATTACGCCTGGTTTGCCCCAGTCAGGGCGCCGTAACGCTTAA;> ACATACATAAAGTATAAGGCTTGCTTTTGCGGGAGGGAAAAT;> TTTTTTTTTGGCACCGCTTCTAAGCCTTTATTTTTTTTTTTT;> TAGTGGATATGGTAAACTTAGGCAATTTTAAGGCTGGCTGAC;> TGTTGGGAAAATTCAGGGAAGTAGGTACAAATGTAATGAAAC;> TTGAGGGATATGGTTGGCTCAAGAAATGTTCACAGTTCAACT;> CCAGTTGCTGACCACCGTAATCAGTACCTTACTTCGGGGGTG;> GCATGTCTCATTAAATAACGTTGCGCCGCTACAGGTTTGGGG;> TTTTTTTTTTTGAGGGGACGACGCCGACTTGAGCCATTTGCT;> AGCAGCAGTTAGAAACAGGAACCATCACGCAAATTCTAAACA;> ACCATTACCTGTTGTTGCTGGGTAATAACATCACTAGCACGT;> TGTAGCGGTCACGCGAACGTGAATTTGAACGGGGTGTAAAAC;> AAGTTTTAGGAAGGTGGCAAGTTTCATTGCAACTACTGTAGC;> TCCCTTACGAAAAACCGTCTACCAAATCGATAAAGGCCAGAA;> TTGGAAATCAGGAGCACTTAGATTAGGGGTAAATAAATCAGA;> CTTGGCTTCTAGGTCATTGAAATACACAATGTAAGTCAGAAC;> GAGTGACTCAAACAAGGAAGCGGCATTAAAAGGTACCAGAGC;> TTTTTTTTTAGGAGGTCCCTGATCTAACCCTTTTTTTTT;> TTTTTTTTTCTACGTGAACCATCACTCAGGGCCGAAATC;> CACGACTTGACCCTTGAGGTCTGTAGTGTTTTTTTTTTT;> TTTTTTTTTAATTCTACCGATGGCCCATTTTTTTTT;> TACAGGACCATTATCATCAGAAGGCGGATAAGTAAAACGCCG;> GGAACATACAGTGCCCATATCGAAGCAGTGGATTATACTTCT;> TTTTTTTTTAATCAGCTCATTTTCCCCTGCCTATTTCGGATG;> CTATCTACTCAAGACGTACTCGCCCTCAAATCCATGCCCAAT;> TAAGTATTTTTGCTTTTATCCAACCACCACACCCGAGCTTGA;> GATAGCAAGGAGGTGAAGATGACTGATGAGAGAGGCGAATTA;> TTTTTTTTTAATATTTAAATTGTAACCGCCACCCTCAGAACA;> TGATAGGCAGTACACCGGCTTGTAGAACCAGTGACAGATTGT;> AAAGTAAGTGCATAGCTTAGATTGTCCAATCCAGTGCGCGTG;> GCTTACACACAGCCTATAATGAAGTACGGTTTAGACAAACAC;> AGTCAGGTGGGTCTTGAGTTTGAAGCCTAATTGCCAGTGGTC;> TCGTCACTATACTGTTATTGTATGGAAACAGTACAAATTACA;> AGGAACCGTTAGCGTTAGAGATGTACTTCTCTCCAACTTTGA;> CACCTAAGTTTCCCACCCTCTATCTAATCCAAGGATAGGGCA;> AAGCTAGTGCTAAAAAAAAGATAGTATCCACACACACCTCCA;> TTATGGGCATCCAGCTAAAGTATAGCAATAGTGCCACACTTA;> TGGAATCGATTTTGCCTCATACATGTACAGAGCCATAGCTTA;> CTGTATGGGATTACTATTAGTAAATGAATTTAGTTAATTTGA;> CAGAGGGGTGTAATAGGGAGTTATATAATTATTGCAACTGAT;> AAACAACAGCCAACGCTCACTCCCATCTTCTGACCTAAATTT;> ACAGTTTCATAATTTGGTTACTGTTAGCTACATCATACCATG;> ATGTGCCAGGACATCCGACTTGGTTCACGAACTCATCTCCAA;> CTATACTATGGCTAGAAAGAGATTTGTACACAGCTTAGAAGT;> CTTTTTCATGAGGAGGCTTTGTGTAGAAAATATCCCATCCTA;> TTTAATGTGAAGTTATACTGCAGCATAATACCCTATCTGATA;> TTTTGTGCTGTTCTAGTAGCTTGCCCATTGCTCCAAGTCAAC;> CGGATATACCAACTAACAACAATGGTAGTCATCGCAGCCTTA;> TTTTTTTTTCAACGCAAGGATAGAACCCTCATATTTTTTTTT;> TTATACCTTATGCGTTGGGGCCAATAGCAGGCTATAAAATCA;> CAAGCCAGTTAATGAAGGGACTTACCAGATATGACCCCCGAT;> CGTGACCCCCTCTTCTCAGCAAGGTAGTCTGGCATAAATCCT;> ATACATAATATGCACAGATCTGATCCTGACTAGGATGTACTC;> TCATCAGACAACATTATTACAATAAAACCATACACGAGTTAC;> TTTTTTTTTGGGTGTGCCTCATAAGGCTTATTCTTATGCAGC;> AGGCATATACCCATATCTCCTAATACACTAGCTTTACTAATT;> TTTAGTCTTGAGAAGGCTAAAGAGGGTTAAGGTATCTACTAA;> CTTCTGTCAAAAGGAATTACGAATGCAGCTTCATCTATGGAT;> AACCAAACCCTCGTTTACCAGGAAAGATCCAAATCACACTCT;> CGATAAACTCTTCAAGGGAACACCCACACCAGAGTACACCAG;> AATAGTAAAATGTTTCATAAAATGAATAAGCGAAACAAGAAC;> TGAATCCAGGGGGTGATCTCCCAAGAAGCTAAAACCTATGAA;> TAACTTGGCTGAGGCCAACTAGGAAACTACGACAATAAACAA;> TGACCATAAATCGAAGGTTCAGAAAACGAGCTTATCCTTTTT;> TTGCATCAAAAATTCACGTTGGTACAACAACCAGCCCGACAA;> AAGCGGATAGTTTGGCTCTCCGGAATCGTAGACTGCTTGTGA;> TATAGTCAAATATCACTAAAGTATAAGGGTACCTTTGCTGAA;> TTTTTTTTTTTCATTTGGGGCGCAAAAATCAGGTCGCTTCAA;> AATATAGGCCCGAAAGACTTCAGAAGCAAAAGGCTACAATTC;> TGACAAAGCGTTTTAATTCGATTTACCCTAATTGTATGAAAG;> ACCGGAAGCAAACAAAGATTTGCGGAGTTACAAATCTCCCTG;> CAGAGACGTGCTACGTGCCAAAATAATTTCATAATATCAGTA;> TCCTTTTCATTCAATCTATGCAGTAGTTAGGCCCTACAACTA;> CAGAGCCCTTTACACAAAAGGAGTAACATTATCAT;> CACCAGAAACTTCCACAGGACGTTATTAATTTTAA;> GGAGACATATGAGTCCCTAAAGGGAGGCCAGGAAC;> CCTTGTGAGGTTGAACCGGAAAGGCCATCTTTTCA;> ATAGAGTTCTGGATTTCAATATTGACAATGAGAAG;> CTGAGTCTCTGAATTCATCATGCTTCAGGGAGGCA;> TGTACAGAGGTACTTAATTCAGAAGTGTATAGAGG;> TTGAGTAGTGTACTTGCGTAGAGCAGGAATTCTCA;> CAGGTTCAGCGGGGAGCCCGGATTGATTGAGAAAC;> CAGTACCTCCTAAATCTGTGAATATACAGTAACAG;> TTTTTTTTTACATCTCACCTCTTTACCTTTTTTTTT;> GTGGACTCCAACGTGGTGGTTAATACCCGAACAAA;> AACAGAGATAGAACCAGAACAATAAAAAAATTAAA;> GCTGGATGGGACATATGGAAAACGAACCACCAGCA;> CTTGGAGCACATAGGAATACTCTCAGTTCCTGTTT;> TTCAAGTGCTGTAGGTGGCATTAAAACATATCAGA;> ACAGAAAGATGACATTTAAATTTTCAAATCCCTGG;> TTTTTTTTTGCTCACTGCCCGCTTTCGAGAGCCAG;> AAATTGTCCACAAGTGAAGGCTGTCCTACCGTAAA;> TTTTTTTTTAGCCGGAAGCATAAAGTGAGGATTTA;> TCCTTTGATTATCATGGAAAGTTGAGTATACTGCT;> GATGATGATCAGTGGGCCTATGCAATTAAAAATTA;> AGGAACACTGCACAATTTTCAGGTTTCTTGGATGA;> TTTTTTTTTTCGTAATCATGGTCATAATCCTGATT;> CTTGGGTAGTGGCTCACAAGGGATGTTCCAGGAAC;> TAACACCCTGACGCAGTGGTCATGGTAAGGAACGT;> GAACCTACCGTATACATTAAATAATATTCACAAAC;> GCTAGTCGCAGGATCTTCAATAACCCCCGATTTAG;> GTGAGTGCAAAATTTAAATCATGTGGCCTGCATAG;> AGGTTATGGAGTGTTTTTGCTCTCTGTAGCGAGAA;> GATGAGTCCTCTTGTTGAGTTGCCTGAGCCTTACC;> TGCTTCTGTAAATCAGCAAAATTAGTACAGAGGCT;> CCCATATGCCCTAGAAACAAAGTGACCATGAGGGA;> CTTAATTTTCCCTTAGAATAGTACCGCCACCCTCA;> ATCATAGGTCTGAGGTTATATCTGAGTTATTCCAC;> TAGATTAAGACGCTAGACAAATTCAGGGTTTGTCG;> AATCGCAGAGAAGAGATGCACCCCCTTGAAAACAT;> AATAAGGCGTTAAAAAAAGCCAAGGAATCCAAAAA;> TGAAATACCGACCGTGCGTTAGAGAATAGAGCCTT;> GCCACAAGTAATAAGAGAATACCAGACGAGAAGAG;> TTTTTTTTTATGGGGTGGTGGAGCTCTGCTGACCT;> TTTTTTTTTGTGATGACTCTGATGGTCAAAGCAGA;> TGGAGGAGAGATTTCCTCCCAATGATTCGCCCAGT;> AGCCCTATGCATATACCAATCTAGCAAGTATGGTC;> CAAATCAGATATAGACGAGCAAGGACTAGCCGACA;> AACTATGTCAATTAATTGCAGGCGGGAGAAACAGC;> TTTTTTTTTCTTATTAGTTGCTTAAGCCACCTGTT;> AGGTTGCATTGACTCCACATACAATATACCATAGT;> GCAGCCTCTACCTATTGTAGGTTTATTAGAAGATG;> TTTTTTTTTGGCGATTAAGTTGGGTAATCCAAATA;> ATTAAGTGCATTAGGGAGAGTAATCTTACCAACGC;> GTCAAAAAGTTAAGGACGGTCCAAAGCTGCTTTTT;> TCTGAGTGAGCTCCGACTCTTTCATTAGAAATTCA;> GATGTTTATATCAGGAGAGAATTACTCTTTACTAG;> GAGCATGAGAATTGATGAAAATGCGATTTTTTGTT;> TTTTTTTTTTTGGGAAGGGCGATCGGCAATAATAA;> TGCCCACCTACACAATAAATCAAAAGAATTGGAAC;> CGCAATACATTTTATTAGGAACGCCAAAGACAAAA;> TAGGAATGACTGATTGTGTAACAGACTTGGAAAGC;> TCATAGGAATGCTCTGGAATTTTGACTATTCACCA;> TTGCGACAGAATCATCCATGAAAAGATCAAATCAA;> TTAACAGGCCCTAGTAGAAGGGATTGCAGCCAGGA;> TAGCTGTTTCCTGTGTGAATTTTTTTTT;> GGGGATAAGAAATATACCTTTAGCTGGC;> GAATATACCGAGCTCGAATTTTTTTTTT;> CAGATGAGTCTTGGAGGAGAAATTTCAT;> CAATAACGGCAAGATGAGGGTATGAAAC;> ATACCACCTCGATAAAGACTTTTTTTTT;> GCACCGGCTATGTTGGACCTTTGGCAGA;> TTCATACAGGGCTTAAGCTTTTTTTTTT;> TTGAACAACGCCGTCGAGAGGTAGAACA;> AGCGACATTTCACATAAATTTTTTTTTT;> GAGACTCAGGATAATGCCCAGGGATTCGCCTGATT;> AAAATCTTGCGAATGTGGAATACCTTATCTGTAGC;> TCTTAATATAGGATAGCTAATGCAGAACTAATTTA;> AAGGCCGCTACTGGGAAGCTATAAAGTAATTCTGT;> ATGACAACTTGATAACAAGAATTTATCAACAATAG;> CGATTATATTTTATAAGCCCCACTTGCATTGAGGA;> TCTGAATAAAGTACGCTATTTTCTCTCAGTGTTTG;> TCTAAGCTGAATAGCTACCTCAGTATTTTTTTTTT;> CTTGAAAATAGACAACAGATTGGCATGGAGACCAC;> GAATACAAACGTAAAATCATATGGCCGGAACGAGG;> AAAAATCATTTCAGGCTGCGCAACTGTTTTTTTTT;> TCCACAATAAAGTCAAGAGTAATGAACGTTTGCTG;> GTGCATGGATACCTCCTCTAGACAACCCAGGTAGC;> GCTGTACCAATTATTTTGTACTGGCTTTTTTTTTT;> TTTTTTTTTTACCCAGTCAATAGTAAAAGTCCTAA;> CATGCCTTGCTACTTTGACCCGGATATAATACCAG;> ATACTCTAAAAATACAGACCTTTGAAAGAGCGCTA;> TGTGTATATGTTGGTAATCACTTCTTTTTTTTTTT;> TAAACCATGTAGCAAGGTGCTTGCGGGAGTACCGC;> GGCCACATTTAAGACCCAGCAATTGGTTTTTTTTT;> TTTTTTTTTATTGGTGTGGTTTGTGTTTAATAAGT;> GATAAGAGGTCACCACAACGCGGTTGCTAAGTCAG;> GCTTAATTAATTGCAGACAGCATTTGAGGTTCTCA;> CTACAGGATTTAGTTTTCTGGAGGGGGTCTGTACT;> TTGGGGTCAAAGGGTAAATCAATGTGCGTTTTATC;> AAAGAACGATAGGGAATCAATAAGGTAGAAGGATG;> TAATGATAACTCGATATTTTAGGCAAAATGACAGG;> ACCTTCTTAAGTAGGTATTGTATTCTAGCAACCGA;> CAATGCAAGAGAGGTGAGTAGGCCTAGGAAACTGC;> AGGTGAAACCACGGGTGAGAAACACCAGAACGA;> ACTGTGCACCTATGAGGAAGAGGGGTTCCCAT;> TTTTTTTTTTCTGCTGTCCTTATCATAAGTAA;> AAGAGTCCACTATTATCCCTTCTGGAAA;> TCACCTGCCCTTCACCGCCTTTTTTTTT;> CTATGTTCACCAGTGAGACTTTTTTTTT;> TAGACAGCGCTAGGGCGCTGGTTGACGG;> TTTTTTTTTGGGTGGTTTTTCTTGTTGC;> GTAAAAGGGGATTTGCAAGGGCGACATT;> GTCACACCATGGAATTTATCTATCACCA;> GGGACATCATTGCATTAAGCCACAAGTC;> TGGCACGGCCAACGCGCGGTTTTTTTTT;> ATGCGCGCGTTTTCCGGAAACAAAGTAG;> GGGAAACCTGTCGTGCCAGTTTTTTTTT;> AACACATTAATTGCGTTGCTTTTTTTTT;> CATTTGGACTAGCCTATGATGAAAAGGT;> CAGTTGAAAGGACTGGATCTGCTAGTAC;> TATCTAAGCCAAGCTACTGTGTAATGTG;> TTGTAAAGCCTGGGGTGCCTTTTTTTTT;> CTTAGGGCATTATGCAAGGGCGCCCCTA;> AAATTCCACACAACATACGTTTTTTTTT;> ACCTACTCAGGTGTGGCTTAAGAAACTT;> GGAATTATTACCGTAGTTTTAATCACAA;> TGACTATAGGCCCCCATGAAAGCATAAC;> GCGATTAAGAGGAATATCCTAATCCACC;> AGCGATGTTTAGCTATATTTTTTTTTTT;> TTTTTTTTTAATGGTCAATAACCACCAG;> CCATTAGATACATTTCGCATTTTTTTTT;> GTCAGGATAACGATATCATGTAACTGTT;> CCGCGCTTAATGGAGCAGATGCTTTTAA;> AGCCGGCTGCGCGTACTGTCCATACAGT;> TCTTGTCATGGTTTCGCCAAATTGAGTG;> GCCAGGCGTCACCAGCCACCAATATTAC;> GATGAGTCTGGAGTCAGCATTTTTTTTT;> AGTAATCCTGGAGAAGTAATTTTTTTTT;> CGACTTTTTCAAATATTATTAAGGAGTC;> TCTTACCAATGGTTCCTGCTGCTTGGAT;> CTCTGGTTATCACAGCAAGTTTTTTTTT;> TCCCCATAGGAGTTACATCAACATGTAC;> TTATTTAACAACGCCAACATGGCGCCTG;> AATACTTCACCCTATATAGTTTTTTTTT;> AAGACCTATCTTAATAGTACTACCCCAG;> GTCCTGACCGATAGATTGAATTTCTTAA;> ATTCCAATAGGTTGTGTGGTTTTTTTTT;> AGCTGGAAGATTGAGAGGCTTTTTTTTT;> AACGCGAGGCGTTTCTTATCCAACGGGT;> AATGGACACCCCACATGGTTTTTTTTTT;> TAAGGGGGATGTGCTGCAATTTTTTTTT;> TTTTTTTTTTTACGCCAGCTGGCGAAAC;> CCTGCGGGCCTCTTCGCTATTTTTTTTT;> CTGGCTGCAGTTGTAGGTTGGCAACTCT;> ACCTTTAAAGGTTGTACTGAACACCCTG;> AGGTTTGGTTACCAGAAGGAAACCGAGA;> GTAAGCAGATAGCCAAAAGAACCAGTGC;> CTGTAAAGAAGGCATGGGCACTGTCACT;> CTAAACGCAAAGACTTATCACCGTCAAC;> TAAGGGCGCTGAGCATACCTACCACCGA;> TTTTTTTTTGCGGATTGACCGTAATGCC;> CAGGACACAAGGATTTAATACGTATGGA;> CTAAATGCCTCCCTCACTAACACATGGC;> TACTCCGTGGGAACAAACGTTTTTTTTT;> TTTTTTTTTTAACAACCCGTCGGATTAT;> TTTTTTTTTTAGCCAGCTTTCATCAAGA;> AACGCGTCTGGCCTTCCTGTTTTTTTTT;> TTTTTTTTTCGCCATCAAAAATAATTAT;> GAATTTCAAGGCAGTGGGTATTGAATGG;> GCCTAAGACCAGCAAGGGTTTCAACACC;> AGTGTTCGTTGATATTTAACATTGGTCT;> CATGCATAATAGGTAAGAAAAGACAGCT;> GAGCCAGATTGTATAAGCATTTTTTTTT;> TTTTTTTTTTGTGTGATGGGGAAAGACT;> ATCGGTTAGTTTCAGTTGGCTTGAATTT;> TTTTTTTTTGATTGAAGTGATTCTCTCT;> ACAGGAGTTGAAAGCATTATTTTTTTTT;> TTTTTTTTTAACAAGCCTACTAGCAGAT;> TTTTTTTTTTTATAACATTCCAAGTTAA;> TTTTTTTTTTAGACTGGAGGTGTGTACT;> CCATGTTACTTAGGCGAAATCCCGACTT;> TTTTTTTTTAAAGATTCAAAAGGGTGCT;> CGCTGAGTAATGTGTAGGTTTTTTTTTT;> GACCAGGCGCATCACTAGTCCTATCAAT;> TTTTTTTTTTATTTTAAATGCAATGCCA;> ATGGGTCTGCAAGATTGAGATATCATAA;> TGAAAGTGGGTATATCAAGTTTTTTTTT;> AAGAAGTACCTGGAGTGTACAAACAAAG;> TAACCCAGTGATAATAGCTGCGCAGAGA;> GGTGAACATTTTAAGAGCATTGCCTCTG;> TTTTTTTTTCATTTCTCCGAA;> TGTTTAGGAAAAGACTTGAAG;> AGTATAATTTCAACTATCAGC;> TTTTTTTTTTCAGGATTTATG;> CCGGAAACCAGGTTTTTTTTT;> GTGTGGCAACATATAAAAGCC;> AGCCAGCTTTCCTTTTTTTTT;> TTTTTTTTTAGGAAGATCGCA;> AGTATCGGCCTCTTTTTTTTT;> AAGGAATTAGAGCCAGCAAGT;> GCATCTGCCAGTTTTTTTTTT;> CTTTAGCCATCGATGTGCAGT;> TTGGTGTAGATGTTTTTTTTT;> AATTATTGGCAATGTATTAAA;> TAGGATTTTTAATCGGGGTAC;> TTTTTTTTTTTTAGGGGAGGT;> TTGCTTTCGAGGTGGATTGCT;> TGCCACTTCCATTAGGTATTC;> TTGGGCTTGAGATGGTTTA> SAQEPARKKQDPPVTHDLRVSLEEIYSGCTKKMKISHKRLNPDGKSIRNEDKILTIEVKKGWKEGTKITFPKEGDQTSNNIPADIVFVLKDKPHNIFKRDGSDVIYPAR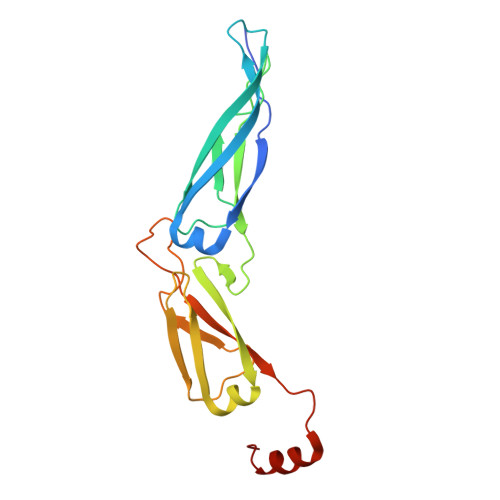ISLREALCGCTVNVPTLDGRTIPVVFKDVIRPGMRRKVPGEGLPLPKTPEKRGDLIIEFEVIFPERIPQTSRTVLEQVLPI> MLRDLFDRAVVLSHYIANLSSEMFSEFDKRYTHGRGFITKAINSCHTSSLATPEDKEQAQQMNQKDFLSLIVSILRSWNEPLYHLVTEVRGMQEAPEAI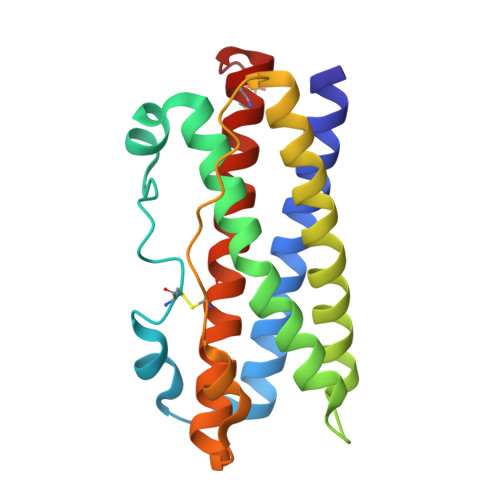LSKAVEIEEQTKRLLERMELIVSQVHPETKENEIYPVWSGLPSLQMADEESRLSAYYNLLHCLRRDSHKIDNYLKLLKCRIIHNNNC> MVMQENHLIDIARWSERPGPRGIPSICSAHPLVIEAAMLRAHREKAPVLIEATCNQVNQDGGYTGMTPEDFTRFVGAIADRIEFPREKILLGGDHLGPNPWKHLPADEAMAKAEAMITAYAKAGFTKLHLDTSMGCAGEPTALPDATTAARAARLAAVAEDAVGGRGGVLPVYIIGTEVPIPGGALEEL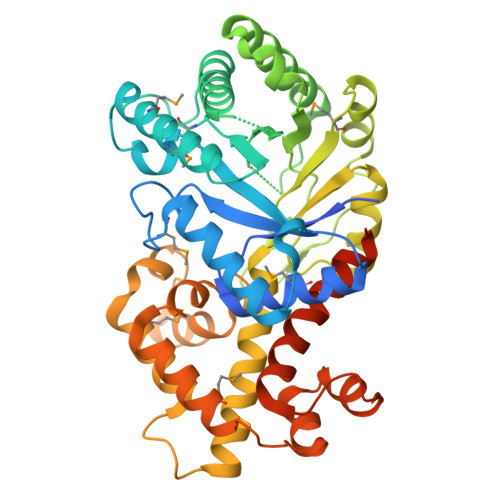DTLEVTAPEAAIETVRVHRAAFEEAGAAGAFSRVVGAVVQPGVEFGNENVIAYDRARAEKLSATLGQLHGMVFEAHSTDYQTPDALRELVADGFAILKVGPGLTFALREALYGLDQIAAFLFPAARERTLAEVTEAVMREEPANWAKYYHGSAEEQRLQRHFSYSDRIRYYWPHPKAAAAVDELMSLLDGVAIPETLISQFLAGSYARVRNGEVAPQAKPLALAAVDAVLQDYFAACRVAENLYFQSHHHHHHWSHPQFEK>MRILADENIPVVDAFFADQGSIRRLPGRAIDRAALA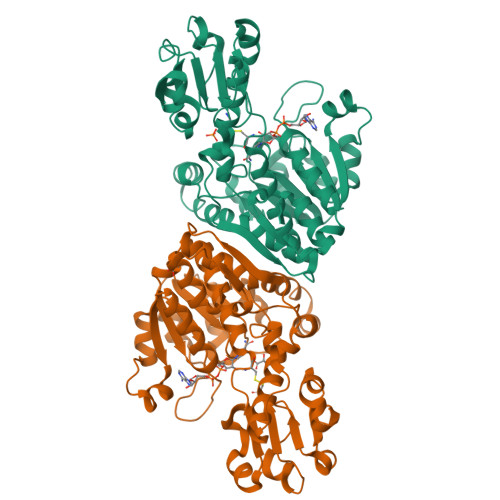EVDVLLVRSVTEVSRAALAGSPVRFVGTCTIGTDHLDLDYFAEAGIAWSSAPGCNARGVVDYVLGCLLAMAEVRGADLAERTYGVVGAGQVGGRLVEVLRGLGWKVLVCDPPRQAREPDGEFVSLERLLAEADVISLHTPLNRDGEHPTRHLLDEPRLAALRPGTWLVNASRGAVVDNQALRRLLEGGADLEVALDVWEGEPQADPELAARCLIATPHIAGYSLEGKLRGTAQIYQAYCAWRGIAERVSLQDVLPETWLAGLQLNPGCDPAWALATLCRAVYDPRSDDAAFRRSLTGDSATRRAAFDALRKHYPPRREITGLRVATGGQAELQRVVRALGAQLV[2x]> MHHHHHHAVRASEISRVYEAYPEKKATLYFLVLGFLALIVGSLFGPFQALNYGNVDAYPLLKRLLPFVQSYYQGLTLHGVLNAIVFTQLFAQAIMVYLPARELNMRPNMGLMWLSWWMAFIGLVVAALPLLANEATVLYTFYPPLKGHWAFYLGASVFVLSTWVSIYIVLDLWRRWKAANPGKVTPLVTYMAVVFWLMWFLASLGLVLEAVLFLLPWSFGLVEGVDPLVARTLFWWTGHPIVYFWLLPAYAIIYTILPKQAGGKLVSDPMARLAFLLFLLLSTPVGFHHQFADPGIDPTWKMIHSVLTLFVAVPSLMTAFTVAASLEFAGRLRGGRGLFGWIRALPWDNPAFVAPVLGLLGFIPGGAGGIVNASFTLDYVVHNTAWVPGHFHLQVASLVTLTAMGS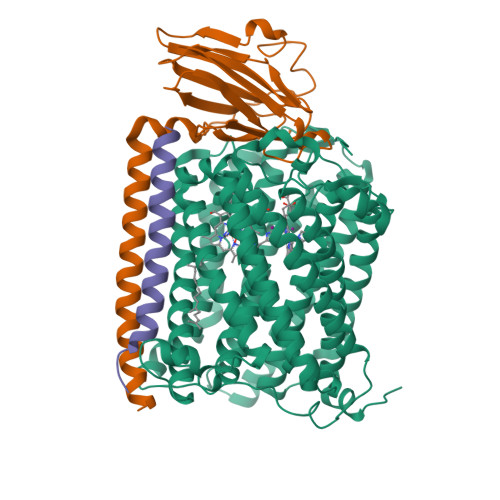LYWLLPNLTGKPISDAQRRLGLAVVWLWFLGMMIMAVGLHWAGLLNVPRRAYIAQVPDAYPHAAVPMVFNVLAGIVLLVALLLFIYGLFSVLLSRERKPELAEAPLPFAEVISGPEDRRLVLAMDRIGFWFAVAAILVVLAYGPTLVQLFGHLNPVPGWRLW;> DEHKAHKAILAYEKGWLAFSLAMLFVFIALIAYTLATHTAGVIPAGKLERVDPTTVRQEGPWADPAQAVVQTGPNQYTVYVLAFAFGYQPNPIEVPQGAEIVFKITSPDVIHGFHVEGTNINVEVLPGEVSTVRYTFKRPGEYRIICNQYCGLGHQNMFGTIVVKE;> EEKPKGALAVILVLTLTILVFWLGVYAVFFARG> MRSIITQICNGVLHGQSYQSGSNDLDKGNSEIFASSLFVHLNEQGKEIIKHKDSDDKIVIGYTKDGMAFQIVVDGFYGCERQAVFSFIDNYVLPLIDNFSLDLTRYPDSKKVTESLIHTIYSLRSKHAPLAEFTMSLCVTYQKDEQLFCAGFGIGDTGIAIKRNEGTIEQLVCHTEVDGFKDAFDNYSSANIDLVIERNSVFNTKV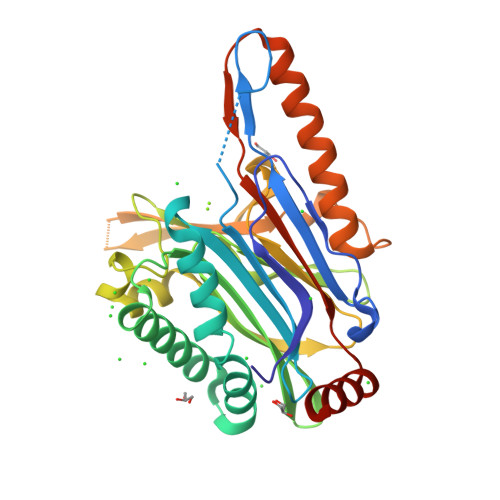MPGDELVGYTYVPPMLEMTEKEFEVETVDGKKINKRIVRHLNLDPGNFDDKDPLFSQLLQVVKSKQKQLVEQAKETGQIQRFGDDFTVGRLVIPDQLLINQLRIHALSHHHHH> LYC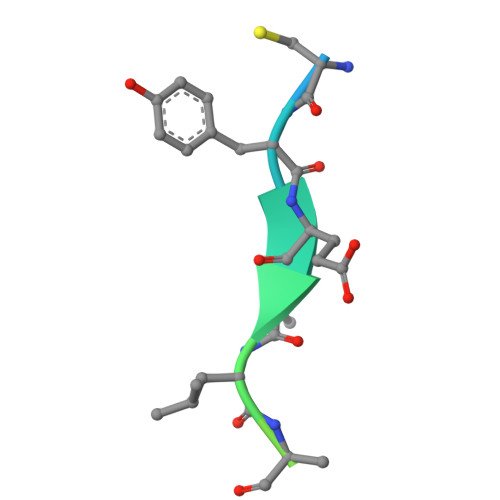YEQLNDSSEEEDEID> MKPHPWFFGKIPRAKAEEMLSKQRHDGAFLIRESESAPGDFSLS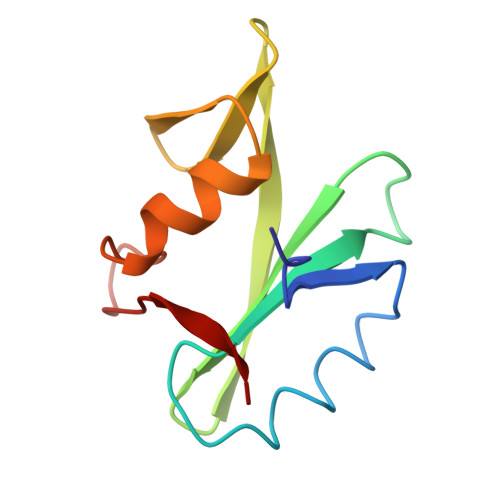VKFGNDVQHFKVLRDGAGKYFLWVVKFNSLNELVDYHRSTSVSRNQQIFLRDIE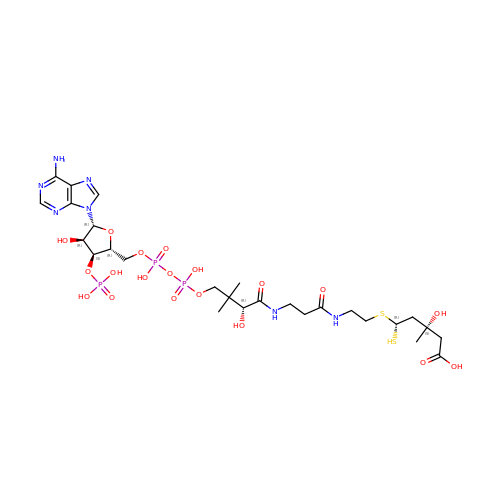(3R,5R,9R,19R,21S)-1-[(2R,3S,4R,5R)-5-(6-amino-9H-purin-9-yl)-4-hydroxy-3-(phosphonooxy)tetrahydrofuran-2-yl]-3,5,9,21-tetrahydroxy-8,8,21-trimethyl-10,14-dioxo-19-sulfanyl-2,4,6-trioxa-18-thia-11,15-diaza-3,5-diphosphatricosan-23-oic acid 3,5-dioxide | C27 H46 N7 O19 P3 S2 | YDFKRXILVYQATJ-NLYQEGKRSA-N> EPCCDSCRCTKSIPPQCHCAN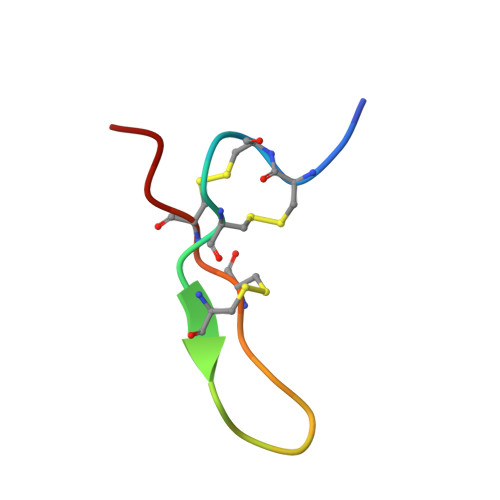I We designed helical heterotrimers with specificity conferred by buried hydrogen bond networks and large aromatic residues to enhance shape complementary packing. Crystal structures of a helical bundle heterotrimer and extended versions, with helical repeat proteins fused to individual subunits, showed all three chains assembling in the designed orientation. We succeeded in determining three high-resolution structures for DHT03: the original base construct, a one-arm version (1arm_A21/B/C) and an elongated two-arm version (2arm_A21/B21/C long). We show that computational design can create cooperative ABC heterotrimers that can assemble as free-standing helical units or as hubs in larger designed assemblies.

The first crystal structure was determined to 2.35 Å resolution. The design model (shown in darker colors) has an overall 2 Å Cα root mean square deviation (RMSD) agreement to the crystal structure (shown in lighter colors) with the largest deviations upon individual chain superposition in chain C. Many of the hydrogen bonds in the design model are not present in the crystal structure, but the overall placement of these residues is relatively close in space to the design model and the ABC heterotrimer still assembles with buried polar groups in the core (water molecules were not detected in Fo–Fc maps, but we cannot entirely rule them out as the overall completeness of the dataset was ~75%). The placement of these residues also appears to be effective in specifying orientation as the chain C orientation in the design model matches that of the crystal structure. There are two possible explanations for the deviations in the hydrogen bonding between the crystal structure and design model. The first is that optimization of nonpolar packing in the actual structure distorts the protein slightly so that many of the designed hydrogen bonds do not form. In support of this, the crystal structure has lower Rosetta-computed energy than the design model due to improvements in sidechain rotamer preferences, Lennard–Jones/van der Waals interactions and solvation energies. The second possibility is that, in solution or neighboring low-energy states, small backbone adjustments allow for more or all of the designed hydrogen bonds to form (Rosetta may not accurately capture the energetic cost of buried unsatisfied hydrogen bonds). On the one hand, the crystal structure of DHT03 shows that many of the designed hydrogen bond network residues are not making hydrogen bonds due to small local distortions in the structure. Instead, they appear to be buried without making any hydrogen bonds, which is expected to be extremely destabilizing.

> GSSPEEEKLKELLKELKKVLDRLKKILERNDEEIKKSDELDDESLLEDIVELLKEIIKLWKILVELSDILLKLIS;> SSPVDEIDKEVKKLEEEAKKSQEEVERLKQEVEKASKAGLDHEGDSRIFKKIHDVVTKQIKVIIRLIEVYVRLVEIIL;> GSKQKEAIKVYLELLEVHSRVLKALIEQIKLFIELIKRPDEDLADKVRKSSEELKKIIKEVEKILRKVDDILYKVKS>[2x]GGGUGAUUAGCUCAGCUGGGAGAGCACCUCCCUUACAAGGAG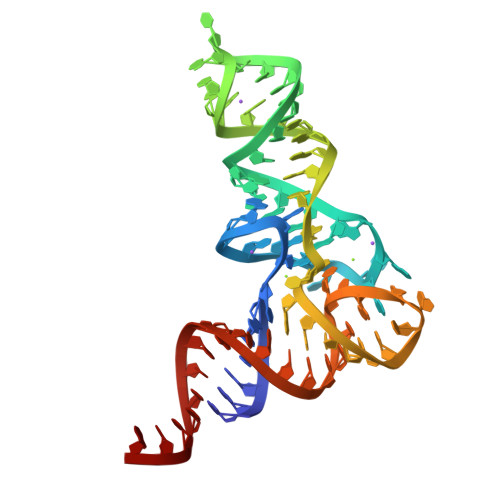GGGGUCGGCGGUUCGAUCCCGUCAUCACCCACCA> TLLEEKVKLEEQLKETVEKYKRALADTENLRQRSQKLVEEAKLYGIQAFCKDLLEVADVLEKATQCVPKEEIKDDNPHLKNLYEGLVMTEVQIQKVFTKH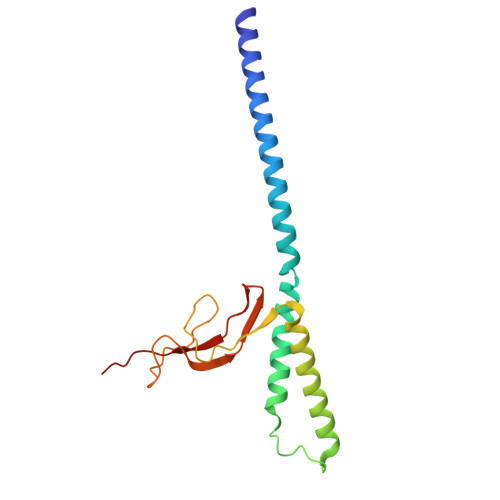GLLKLNPVGAKFDPAEHEALFHTPVEGKEPGTVALVSKVGYKLHGRTLRPALVGVVKEASA>[2x]MLLAHISDTHFRSRGEKLYGFIDVNAANADVVSQLNALRERPDAVVVSGDIVNCGRPEEYQVARQILGSLNYPLYLIPGNHDDKALFLEYLQPLCPQLGSDANNMRCAVDDFATRLLFIDSSRAGTSKGWLTDETISWLEAQLFEGGDKPATIFMHHPPLPLGNAQMDPIACENGHRLLALVERFPSL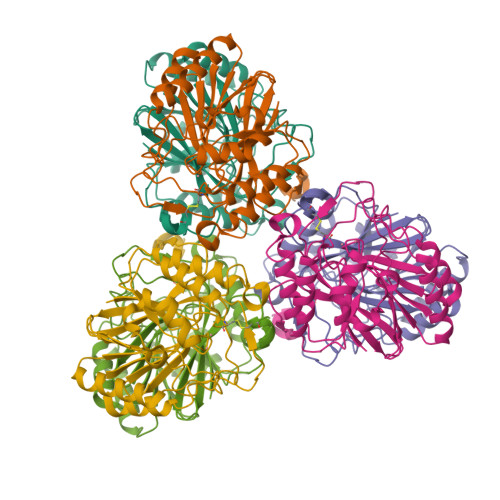TRIFCGHNHSLTMTQYRQALISTLPGTVHQVPYCHEDTDPYYDLSPASCLMHRQVGEQWVSYQHSLAHYAGPWLYDENISCPTEER>[2x]MKPHNSEKYFVKNGQPHFLISGEVHYFRINPKLWRNHLQLLKQTGADTVSTYIPWDWHEIEEDDFDFEGKTHPARNLIRFIKLCKEENLDLIVKPGPYILAEYENQGLPSWLLKKLSKNAFALDENGNVISPDLVSYLSDEFLEYTFKWYDKVMPIISKHQKEHYGPITMMQLCNEIGVFQWLSGKSDYNPKVINLYKEFIIQRYKTIEKLNSVYSTNYNSFDDLKAPSGKIKLRSDYCAYFDFHLFFREYYNKYISILKNKIRSFGINIKLTHNIPGWIYGNASELPMLISTYSEIMKNHPDIIFGLDHIPEFVSFRNAHSDLACNKILEAMQPEAPVWAAEFQAGTREHHVKAY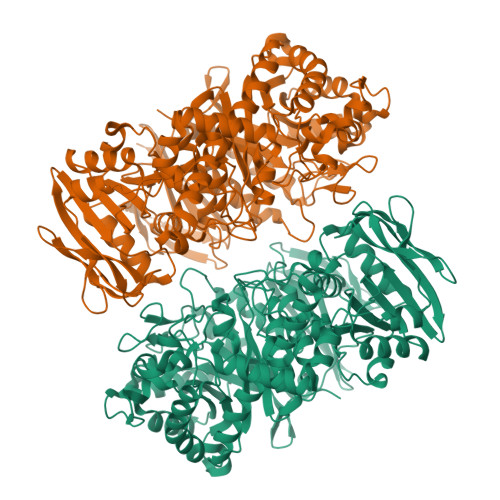AKDLETFYIASLAHGIKGFNYYMFSQGINPEGKGFYGKTFYFQTALDAASNKLALYDSIKKVNRFIRKEQKDLLRTNVNSEICVGFYKPYFFTELISSQLLKEKKLNVEELGLYIDPRFLREEILFNGLLRGLQTLNYNYDVVDLENCDLKSLTAYKQLWITSAEFMDAETQNLLSEFVLNGGNLILYPAVPTLDNYLNRCEILKNNFGIEFITKDSSHKVSAFGIEDVFTAFSKKQIYNDTNSKPIAFTQENEICGIRKKIGKGELTILGFAFGYTSDEHLELIDKLVKLNKIKRELFVSDKDIQFVVRENNKSRYIFFLNYHNERKTFNYRKSSELKKKKSEEISIAPFSYKVIKENKLEHHHHHH>[3x]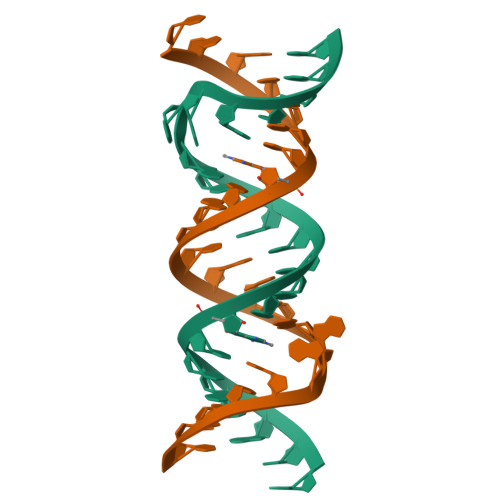UUGCGUCACGUCGACGAAGUCGC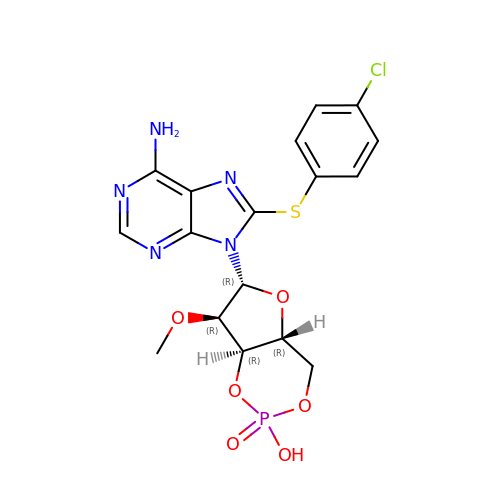(2S,4aR,6R,7R,7aR)-6-{6-amino-8-[(4-chlorophenyl)sulfanyl]-9H-purin-9-yl}-7-methoxytetrahydro-4H-furo[3,2-d][1,3,2]dioxaphosphinin-2-ol 2-oxide | C17 H17 Cl N5 O6 P S | BCGHHRAUZWOTNH-XNIJJKJLSA-N> GSHMRNVAAEQQLRELESTFDGRLGFVALDTA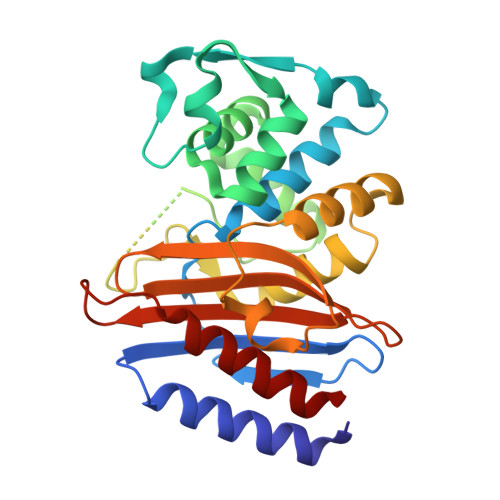TGARIAHRADERFPFCSTFKTMLSAAVLARSAGDAALLQRRIPYAKRDLVRYSPITEKHVGAGMTVAELCAATLQYSDNTAANLLIALLGGPQAVTAYARSIGDATFRLDRRETELNTAIPGDERDTTTPAAMAASVRRLPGDERDTTTPAAMAASVRRLLVGDALGTAQRAQLNAWMLGNKTGDARIRAGVPAGWRVADKTGTGDYGTGNDIGVAYPPDRAPIVFVVYTTMRSRNAQARDDVIASAARIAARAFV>MGALARALLLPLLAQWLLRAAPELAPAPFTLPLRVAAATNRVVAPTPGPGTPAERHADGLALALEPALASPAGAANFLAMVDNLQGDSGRGYYLEMLIGTPPQKLQILVDTGSSNFAVAGTPHSYIDTYFDTERSSTYRSKGFDVTVKYTQGSWTGFVGEDLVTIPKGFNTSFLVNIATIFESENFFLPGIKWNGILGLAYATLAKPSSSLETFFDSLVTQANIPNVFSMQMCGAGLPVAGSGTNGGSLVLGGIEPSLYKGDIWYTPIKEEWYYQIEILKLEI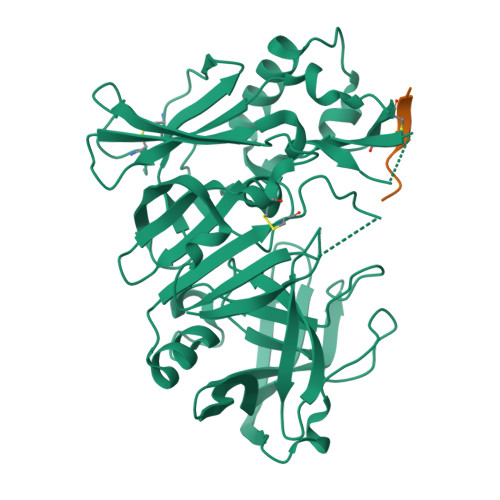GGQSLNLDCREYNADKAIVDSGTTLLRLPQKVFDAVVEAVARASLIPAFSDGFWTGSQLACWTNSETPWSYFPKISIYLRDENSSRSFRITILPQLYIQPMMGAGLNYECYRFGISPSTNALVIGATVMEGFYVIFDRAQKRVGFAASPCAEIAGAAVSEISGPFSTEDVASNCVPA[2x]>GAAUUGCGGGAAAGGGGUCAACAGCCGUACAGUACCAAGUCUCAGGGGAAACUUUGAGAUGGCCUUGCAAAGGGUAUGGUAAUAAGCUGACGGACAUGGUCCUAACCACGCAGCCAAGUCCUAAGUCAACAGAUCUUCUGUUGAUA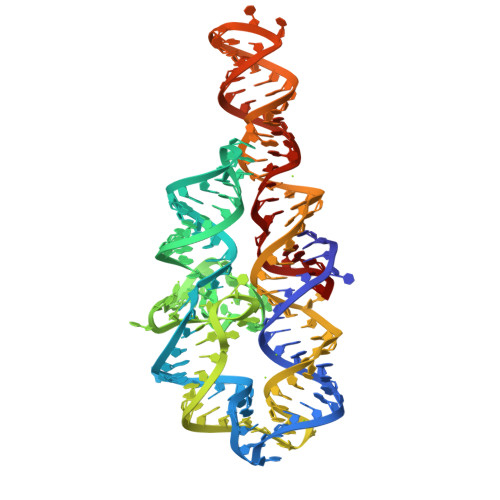UGGAUGCAGUUC[2x]>MGVMGHNWVLSTAADMQGVVTDGMASGLDKDYLKPDDSRVIAHTKLIGSGEKDSVTFDVSKLKEGEQYMFFCTFPGHSALMKGTLTLKGIPGGAECSVDIQGNDQMQFNTNAITVDKSCKQFTVNLS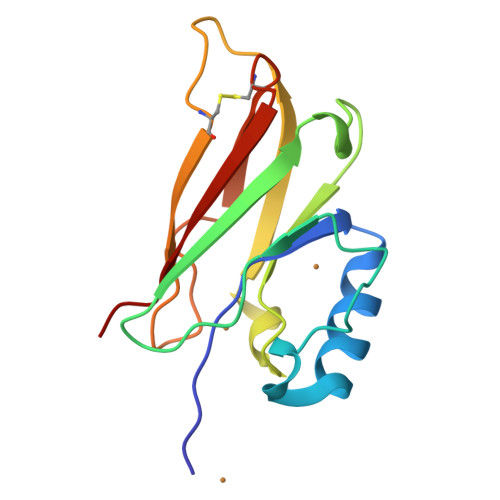HPGN[2x]>[2x]MRGSHHHHHHGSASFLKKTMPFKTTIEGTVNGHYFKCTG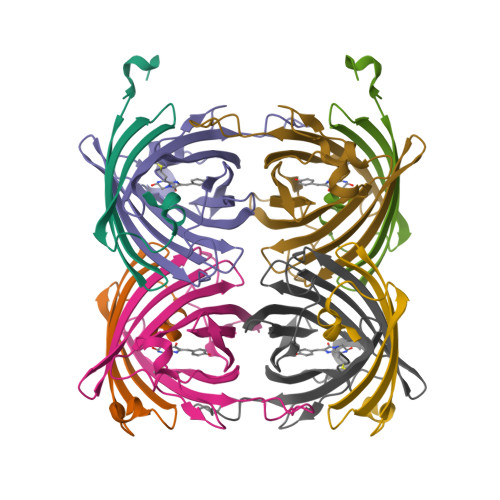KGEGNPFEGTQEMKIEVIEGGPLPFAFHILSTSC;>[2x]MYGSKTFIKYVSGIPDYFKQSFPEGFTWERTTTYEDGGFLTAHQDTSLDGDCLVYKVKILGNNFPADGPVMQNKAGRWEPATEIVYEVDGVLRGQVLMALKCPGGRHLTCHLHTTYRSKKPASALKMPGFHFEDHRIEIMEEVEKGKCYKQYEAAVGRYCDAAPSKLGHN>[2x]MGSSHHHHHHSSMKQAILYVGHGSRVKKAQQEAAAFLEGCKAHISVPVQEISFLELQEPTIETGFEACVKQGATHIAVVPLLLLTAAHAKHDIPEEIVRVASRYPSVRISYGKPIGIDEEVVKAVYHRMKDIGVPYENARVVLIGRGSSDPDVKRDVTGIANLLQEMVPVKEVIPCFLTA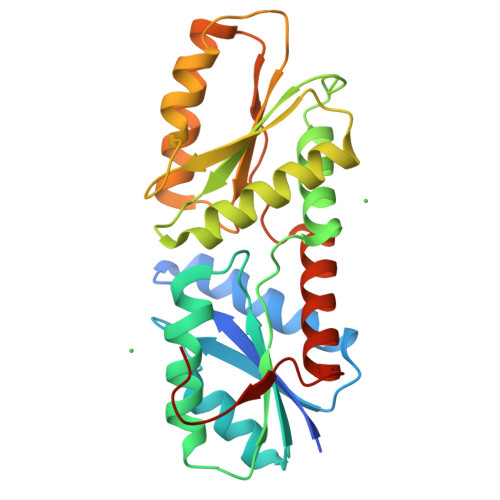CGPNYKEVFSELEKDDGITTFIVPYLLFTGMLMNEIEREVQKLKAHNPNVYLSSYIGFHPHVKNAFLNRVRETAANSEGQFDFDGGSYASAAH CPV are protected by a robust case (polyhedron), each a tiny crystal of viral polyhedrin, whose volume varies from 10−3 to 103 μm3 depending on the CPV type. In the alkali conditions of the insect mid-gut (pH 10.5 or greater), the crystal dissolves to release the infectious virus. The polyhedrins of CPV1 and CPV17 possesses a conserved structural core with modules of variable structure associated with it. Unexpectedly CPV17 crystals contain only a single ATP molecule, positioned in a broadly similar position to an ATP found in CPV1.

In parallel to the XFEL data collection, crystals were analysed at 100 K on a microfocus synchrotron beamline (I24, Diamond Light Source). Data from 768 crystals yielded a moderate resolution data set with a CC1/2 of 0.3 at 2.15 Å resolution. In the absence of a good molecular replacement model, these synchrotron-source data were not, in our hands, sufficient to support structure determination. Using this room temperature structure the synchrotron 100 K structure was solved trivially and refined to 2.2 Å. To accurately determine changes in unit cell dimensions between room temperature and 100 K, powder patterns were collected at Diamond Light Source, which showed a contraction of the unit cell dimension on cooling from 106.1 to 104.9 Å (values used as the cell dimensions for the XFEL and synchrotron analyses, respectively). Despite this temperature-dependent variation in the crystal lattice, the correlation in intensities between the XFEL and synchrotron data was excellent (90.9% overall). The structures are very similar (r.m.s.d. in Cα 0.26 Å after rigid body superposition). To see whether this occurs in the CPV17 polyhedra, we artificially increased the unit cell for the 100 K data to match that of the XFEL data (thereby isotropically ‘swelling’ the structure of the monomer) and performed simple restrained refinement of the resulting structure. Remarkably, these structures were then almost indistinguishable (r.m.s.d. in Cα 0.17 Å). Nevertheless, the strain in the (unphysiological) 100-K lattice is enough to sever the partially formed disulphide bond.

> MADLSLARQRLTDESVNEAPRAYDANMELVIVAEYPEGQCKSFHFANPFVIKGVIKSSELMWDIDNGHQMSEYELQRSINGYAASHSNMRQRSAINRIPKKLSFYLRGNVDWNKASIDIRGPTGLSMRQTEEYSLDRIRPPCSYKRNKFVDLPSCGGRCEKAWYVELDGRPVSIAVIVPRNMHNGINLYAGPLLGNVIEGLDTVPECTQWFDNAPELYAYHASNYGMTMLDQFSVIH N'-[(1S,2S)-2-[(2S)-4-benzyl-3-oxopiperazin-2-yl]-1-(3,5-difluorobenzyl)-2-hydroxyethyl]-5-methyl-N,N-dipropylbenzene-1,3-dicarboxamide 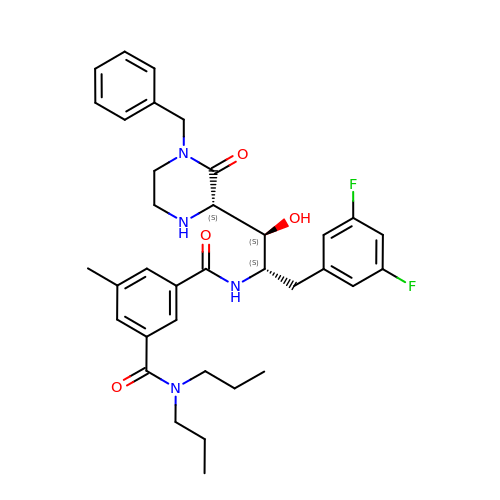| C35 H42 F2 N4 O4 | XKXGRRZAMDHVGR-CPCREDONSA-N> MAHHHHHHMNKQELIDAVAAQTGASKAQTGE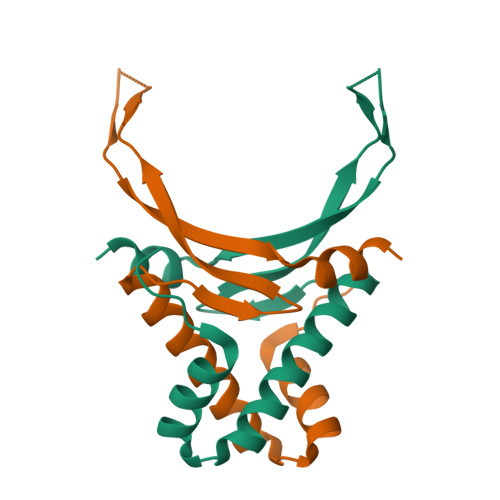TLDTLLEVIKKAVSKGDAVQLIGFGSFGSGKRAARTGRNPKTGETIKIPAAKTVKFTAGKAFKDAVNKR>[2x]TTPSMEDYIKQIYMLIE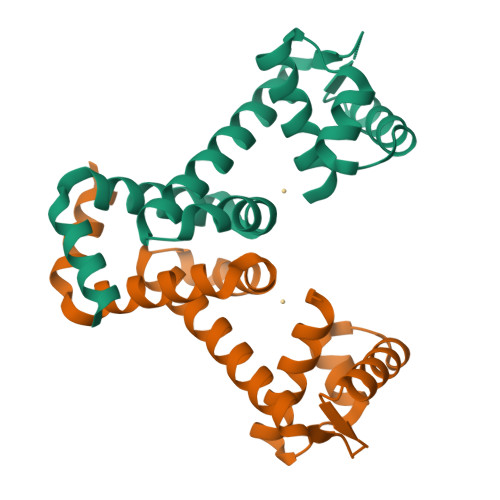EKGYARVSDIAEALAVHPSSVTKMVQKLDKDEYLIYEKYRGLVLTSKGKKIGKRLVYRHELLEQFLRIIGVDEEKIYNDVEGIEHHLSWNSIDRIGDLVQYFEEDDARKKDLKSIQKKTEHHNQ>MSAHRTLLLRLSDSGEPVTSCSYGQGVLTLPSLPLPQGKKLGDMPVYTVKLAIPAGSPVTRDGLIWTNCPPDFSTQFDREKFYKKIIKTSFHEDDHIDLDIYVPGTYCFYLSFKNDKDELETTRKFYFVVLPILSVNDKFIPLNSIAMQSVVSKWMGPTIKDWEKVFARVASKKYNMIHFTPLQHRGESNSPYSIYDQLEFDPTVFKSEKEVADMVERLRTEHNILSLTDIVFNHTANNSQWLLDHPEAGYNHKTSPHLISAIELDKKLLDFSEQMEALGYPVDLKTVDDLIKVMDGIKEHVIGELKLWEFYVVDVKQTVSELREKWGNSKSWSDDNIPSKDDSTNLAQFVRDNATEPGFGSLGERGSNKINIDKFAAILKKLHSEDYNNGIEELATKILNDINLPFYKEYDDDINEVLEQLFNRIKYLRIDDHGPKQGPITKKLPLSEPYFTRFKAKDGEEYALANNGWIWDGNPLVDFASSQSKAYLRREVIVWGDCVKLRYGKGPSDSPYLWERMSKYVEMNARIFNGFRIDNCHSTPLHVGQYFLDVARRVNPNLYVVAELFSGSEAMDCLFVERLGISSLIREAMQAWSEEELSRLVHRHGGRPIGSYKFVPLDDFPYPADVKIDEEYCAYNPDDHSVKCVSEIMIPKTLTATPPHALFMDCTHDNETPNQKRTVEDTLPNAALVAFCSSAIGSVYGYDEVFPQLLDLVQEKRTYSCAENTGISKVKTLLNNMREEIASEAVDIEDSEMHVHHDGQYITFHRTNAKNGKGWYLVARTKFHSSGDQMLPRIKLSQTKATFKAAFSLERTGDAPISDEIIEGIPTKLRELTGFDIGFDENTKETSILLPQDFPQGSIVIFETQQLGIDDSLDHFIRSGAIKATEKLSLESINYVLYRAEQEEYDYSEGRSGAYDIPDYGKPVYCGLQGWVSILRKIIFYNDLAHPLSNNLRNGHWAVDYVVNRLDLYKDKEGVAEVQEWLRSRMERIKQLPSYLVPSFFALVVGIMYGCCRLRAMQLMSDNVGKSTVFVQSLAMTSIQMVSAMKSTSILPDQNIAAMAAGLPHFSTNYMRCWGRDVFISLRGLLLTTGRYEEAKEHILAFAKTLKHGLIPNLLDAGRNPRYNARDAAWFFVQAIQDYVTIVPGGVSLLQEKVTRRFPLDDEYIPYDDPKAFSYSSTIEEIIYEILNRHAGGIKYREANAGPNLDRVMKDEGFNVEVNVDWETGLIHGGSQFNCGTWMDKMGESEKANSVGVPGTPRDGAAVEINGLLKSCLRFVLQLSKDGKFKYTEVTKPDGSKISLSSWNDLLQENFERCFYVPKNKEDDNKFEIDATIINRRGIYKDLYRSGKPYEDYQFRPNFTIAMVVAPELFTPDYAAGAIELADQVLRGPVGMRTLDPSDYNYRPYYNNGEDSDDFATSKGRNYHQGPEWVWCYGYFIRAYHYFNFLTNPKCQVEGSAKKLKPSSYLYRKLYSRLLKHREWIENSPWAGLAELTNKDGEVCNDSSPTQAWSTGCLLDLFYDLWISYEE[2x]

GDE possesses the α-1,4 glucanotransferase (GT) and α-1,6 glucosidase (GC) activities, and removes glycogen phosphorylase-digested branches in two steps56. Its GT activity transfers a maltotriosyl group from the branch to a neighbouring non-reducing end, and forms an α-1,4 glycosidic bond between them. The last residue on the branch is subsequently removed by its GC activity. The structures revealed that CgGDE is composed of four domains, and adopts an elongated structure.

We expressed Candida glabrata GDE (CgGDE, 38% sequence identity to human GDE) in Escherichia coli and crystallized it. A multiple wavelength anomalous diffraction (MAD) experiment using a selenomethionine (SeMet)-substituted crystal gave an excellent electron-density map, which allowed us to build the complete structure. Two very similar protomers were found in the ligand-free crystal. Protomer A contains residues 3–1,528, and protomer B contains residues 4–284, 287–330, 336–341, 345–432 and 442–1,528. Residues 629–651 have the largest conformational difference. In protomer A this region adopts a loop structure. In protomer B this region forms a β-hairpin that contains an inter-strand disulfide bond between Cys634 and Cys645, and sticks out of the structure. The orientations of residues 237–458 in these protomers are also different, and are related by a 6° rotation. Our dynamic light-scattering experiments indicated CgGDE is monomeric in solution, like GDE in other species.6-[2-methoxy-5-(2-phenylethoxy)benzyl]-5-methylpyrido[2,3-d]pyrimidine-2,4-diamine | C24 H25 N5 O2 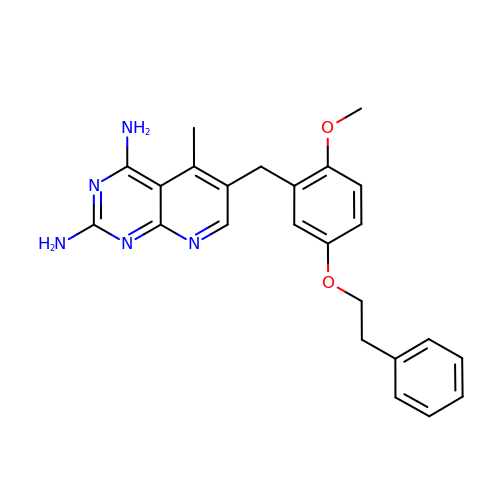| VSDLZXWDJQMRIQ-UHFFFAOYSA-N> MDKCKKVYENYPVSKCQLANQCNYDCKLD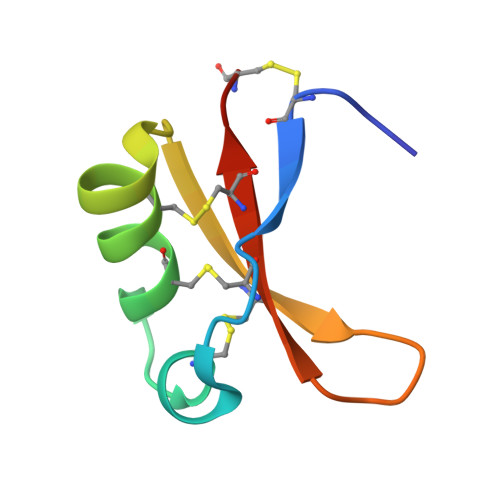KHARSGECFYDEKRNLQCICDYCEY> TLTEDLDAPQDTGNIENGAADNSPQPRTTFDYTGNPLPPDTKLENFFSFYRLLPMGGSGAPSLSFPADEGTIIPLNP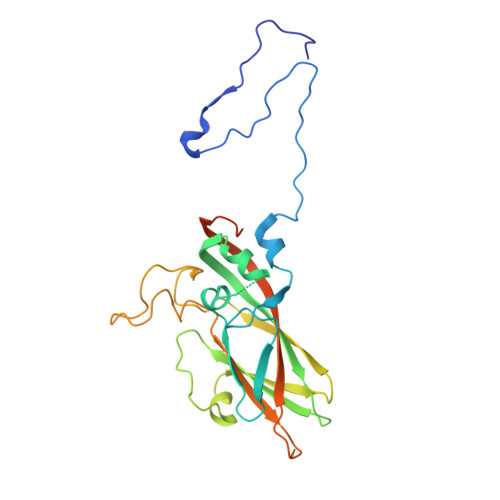INWLKGADVSGIAAMLSCFTYIAADLRITLRFSNPNDNPATMLVAFAPPGATIPLKPTRQMLSNFYMAEVPVSAATSTMVSFSIPYTSPLSAIPTSYFGWEDWSGTNFGQLSSGSWGNLMLIPSLSVDSAIPFDFQLSCWVAFGNFKAWVPRPPPPLPPLPTPAANAERTVAVIKQ>GSPGHMPLSEKGNDPIDSSTIDSLCAAFDKTLKSTPDVQKYNDAINTIFQLR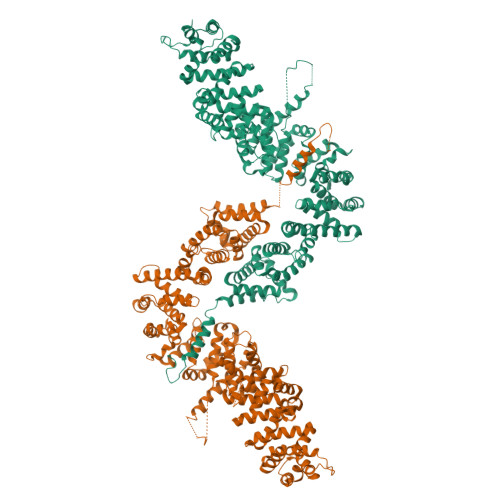QKSESGKMPADLTNSEALKDRQKIEEILTRSYQDHSESRVHLSKLIQNDIPFALNLFEILSRSSIHVFVGCFSNKDATIALLNELQIRIHYGEDTHVTYLLSIILQLLNKFKYNFKEVRFLVKELILRISEDEVKSMMLIIFAELQSSFQKDFDKAVVDFMSSLIVEAEIDVGNDPLSIIVKTLSELYPSLTTLCSEIFLTKGLSKLFKKRVFEEQDLQFTKELLRLLSSACIDETMRTYITENYLQLLERSLNVEDVQIYSALVLVKTWSFTKLTCINLKQLSEIFINAISRRIVPKVEMSVEALAYLSLKASVKIMIRSNESFTEILLTMIKSQKMTHCLYGLLVIMANLSTLPEEXXXXXXXXXXXXXXXXXXXPAADKVGAEKAAKEDILLFNEKYILRTELISFLKREMHNLSPNCKQQVVRIIYNITRSKNFIPQLAQQGAVKIILEYLANKQDIGEPIRILGCRALTRMLIFTNPGLIFKKYSALNAIPFLFELLPRSTPVDDNPLHNDEQIKLTDNYEALLALTNLASSETSDGEEVCKHIVSTKVYWSTIENLMLDENVPLQRSTLELISNMMSHPLTIAAKFFNLENPQSLRNFNILVKLLQLSDVESQRAVAAIFANIATTIPLIAKELLTKKELIENAIQVFADQIDDIELRQRLLMLFFGLFEVIPDNGTNEVYPLLQENQKLKDALNMSLKRGDSGPEFSAAIPVILAKIKV[2x]> MADALGMIEVRGFVGMVEAADAMVKAAKVE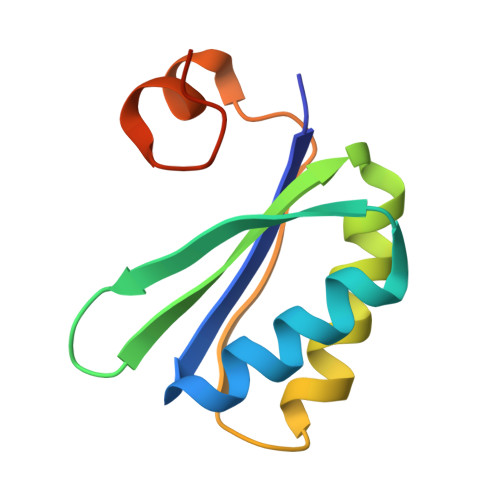LIGYEKTGGGYVTAVVRGDVAAVKAATEAGQRAAERVGEVVAVHVIPRPHVNVDAALPLGRTPGMDKSA> MAHHHHHHNPNYCFAGKTSSISDLKEVPRKNITLIRGLGHGAFGEVYEGQVSGMPNDPSPLQVAVKTLPEVYSEQDE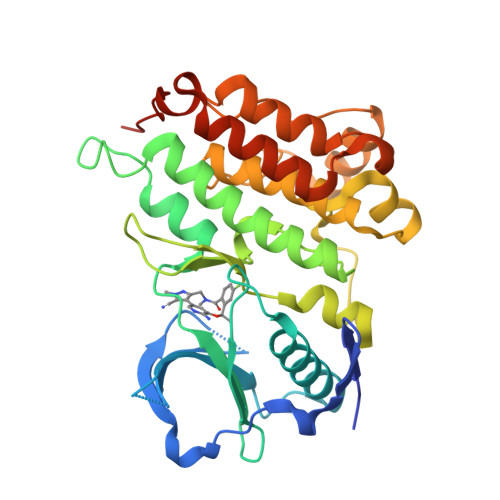LDFLMEALIISKFNHQNIVRCIGVSLQSLPRFILLELMAGGDLKSFLRETRPRPSQPSSLAMLDLLHVARDIACGCQYLEENHFIHRDIAARNCLLTCPGPGRVAKIGDFGMARDIYRASYYRKGGCAMLPVKWMPPEAFMEGIFTSKTDTWSFGVLLWEIFSLGYMPYPSKSNQEVLEFVTSGGRMDPPKNCPGPVYRIMTQCWQHQPEDRPNFAIILERIEYCTQDPDVINTALPIEYGPLVEEEEKV> MHHHHHHMLNRYPLWKYVMLIVVIVIGLLYALPNLFGEDPAVQITGARGVAASEQTLIQVQKTLQEEKITAKSVALEEGAILARFDSTDTQLRAREALMGVMGDKYVVALNLAPATPRWLAAIHAEPMKLGLDLRGGVHFLMEVDMDTVLGKLQEQNIDSLRSDLREKGIPYTTVRKENNYGLSITFRDAKARDEAIAYLSKRHPDLVISSQGSNQLRAVMSDARLSEAREYAVQQNINILRNRVNQLGVAEPVVQRQGADRIVVELPGIQDTARAKEILGATATLEFRLVNTNVDQAAAASGRVPGDSEVKQTREGQPVVLYKRVILTGDHITDSTSSQDEYNQPQVNISLDSAGGNIMSNFTKDNIGKPMATLFVEYKDSGKKDANGRAVLVKQEEVINIANI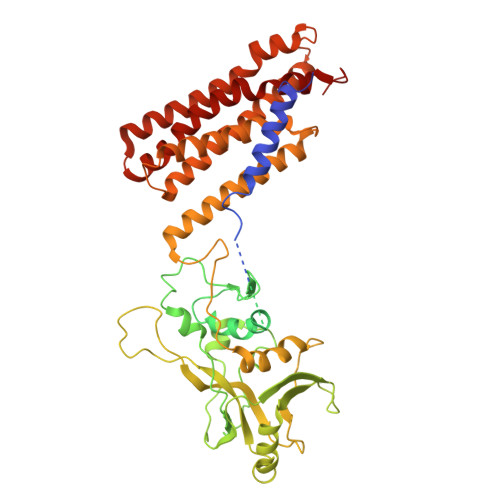QSRLGNSFRITGINNPNEARQLSLLLRAGALIAPIQIVEERTIGPTLGMQNIEQGLEACLAGLLVSILFMIIFYKKFGLIATSALIANLILIVGIMSLLPGATLSMPGIAGIVLTLAVAVDANVLINERIKEELSNGRTVQQAIDEGYRGAFSSIFDANITTLIKVIILYAVGTGAIKGFAITTGIGVATSMFTAIVGTRAIVNLLYGGKRVKKLSI Nsp13 is a highly conserved protein in CoVs and nidovirales and one of the two central components of the membrane associated replication-transcription complex, which performs viral RNA synthesis. MERS-CoV helicase has an N-terminal Cys/His rich domain (CH) with three zincs, a beta-barrel domain and a C-terminal SF1 helicase core. Previous biochemical characterizations have shown that CoV nsp13 exhibits multiple enzymatic activities, which include hydrolysis of NTPs and dNTPs, unwinding of DNA and RNA duplexes with 5’-3’ directionality and the RNA 5’-triphosphatase activity. Our analyses demonstrate that while the domain organization of MERS-CoV nsp13 and EAV nsp10 is conserved, the structures of the individual domains of nsp13 are closely related to their eukaryotic equivalents in Upf1 helicase.

Intriguingly, incubation with a 5’-triphosphate-15T DNA (ppp-15T) greatly improved diffracting power of nsp13 crystals. Next, we collected a 3.0Å resolution native dataset, which we used for final structure refinement and further analysis. There are two nsp13 in the asymmetric unit (ASU) with three zinc ions bound to each N-terminal Cys/His rich domain. Unexpectedly, no additional electron density for ppp-15T DNA could be identified, indicating that a stable nsp13-DNA complex did not form. The CH domain of MERS-CoV nsp13 (residues 1–112) is a compact domain with three zinc-binding motifs stabilizing the fold. The MERS-CoV nsp13 CH domain is tightly attached to the Stalk domain. The nucleotide-binding pocket of MERS-CoV nsp13 is located between RecA1 and RecA2 domains. Sulfate, crystallization condition precipitant, was found bound to the P-loop mimicking binding of the NTP’s phosphate moiety. Residues Gln404, Arg443 and Arg567 from helicase motifs III, IV and VI form hydrogen bonds with the sulfate suggesting their involvement in NTP hydrolysis. Although the helical insertion equivalent to the Upf1 1C domain is missing in nsp13, the protein has a topologically equivalent loop between β17 and β18 which fulfills similar function in RNA binding.

>GPAVGSCVVCHSQTSLRCGTCIRRPFLCCKCCYDHVIATPHKMVLSVSPYVCNAPGCGVSDVTKLYLGGMSYFCVDHRPVCSFPLCANGLVFGLYKNMCTGSPSIVEFNRLATCDWTESGDYTLANTTTEPLKLFAAETLRATEEASKQSYAIATIKEIVGERQLLLVWEAGKSKPPLNRNYVFTGYHITKNSKVQLGEYIFERIDYSDAVSYKSSTTYKLTVGDIFVLTSHSVATLTAPTIVNQERYVKITGLYPTITVPEEFASHVANFQKSGYSKYVTVQGPPGTGKSHFAIGLAIYYPTARVVYTACSHAAVDALCEKAFKYLNIAKCSRIIPAKARVECYDRFKVNETNSQYLFSTINALPETSADILVVDEVSMCTNYDLSIINARIKAKHIVYVGDPAQLPAPRTLLTRGTLEPENFNSVTRLMCNLGPDIFLSMCYRCPKEIVSTVSALVYNNKLLAKKELSGQCFKILYKGNVTHDASSAINRPQLTFVKNFITANPAWSKAVFISPYNSQNAVSRSMLGLTTQTVDSSQGSEYQYVIFCQTADTAHANNINRFNVAITRAQKGILCVMTSQALFESLEFTELSFTNYKLQ[2x]In plants, guanosine deaminase (GSDA) catalyzes the deamination of guanosine for nitrogen recycling and re-utilization. The other involves the hydrolysis of Gua to guanine (G), followed by its deamination to xanthine under the action of guanine deaminase (GDA). Both deaminases are zinc-dependent enzymes, which rely on a catalytic water molecule to attack the amino group-connecting C2 atom to proceed with the catalysis. The zinc ions are tightly bound to the active site, coordinated by the completely conserved residues His80, Cys113, Cys110, and the key water molecule. AtGSDA catalysis needs two key sub-processes: the activation of water and re-capping of the active site, which proceed via the two critical residues Glu82 and Tyr185, respectively.

Furthermore, the Y185F-Gua structure indicated that only one Gua molecule was bound in a substrate-bound conformation but the ligand could be clearly distinguished from the non-reactive state, judged from the rotation angle of the purine ring. It should be noted that these cocrystal structures showed averaged results of multiple deamination reactions, as either the substrate or product could be present in individual enzyme molecules. Accordingly, the C-termini of the enzyme adopted the mixed “in/out” conformations with the last residue Phe185 in the “out” conformer missing. Lastly, the “out” conformer was also observed in the cocrystal structure of the partially active mutant Y185F, and there was only one ligand in the dimeric enzyme. Y185F had difficulties in binding to the substrate, as shown by other single mutants (Y185E/K, etc.) or truncated forms of the enzyme, while retaining the correct fold (as suggested by TSA). The Y185F conformations were reminiscent of the apo-enzyme, where it had one disordered C-terminus in one monomer while that of the other formed loops and pointed out. We found that while WT and Y185F/E showed similar binding affinities toward the ligands, the Y185K and E82Q mutants showed differentially reduced affinities.

>GPHMSDHKFLTQAVEEAYKGVDCGDGGPFGAVIVHNNEVVASCHNMVLKYTDPTAHAEVTAIREACKKLNKIELSECEIYASCEPCPMCFGAIHLSRLKRLVYGAKAEAAIAIGFDDFIADALRGTGVYQKSSLEIKKADGNGAAIAEQVFQNTKEKFRLF[2x]> ATDFRAIMKFDGADSPAMIAISAVLI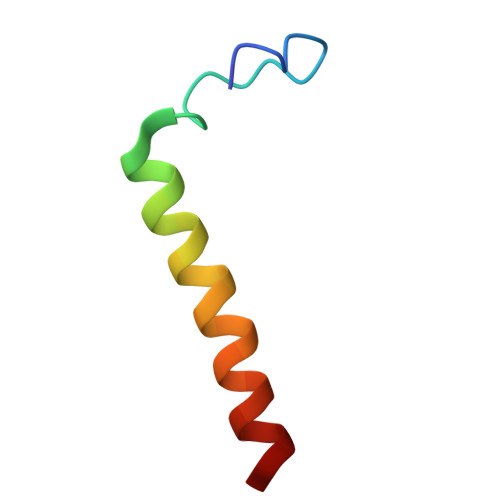LGFIAGLIWWALH>FPIVQVVGFQNSGKTTFIERILEKASEQGLNLGCLKHHGHGGEPQTFTEGKDTDRYQAAGADVTAVEGAGVLQLTARRLWDLTRLIELYQFLETDCLLIEGFKKAPYPKVVILSEKEDLEALKTVN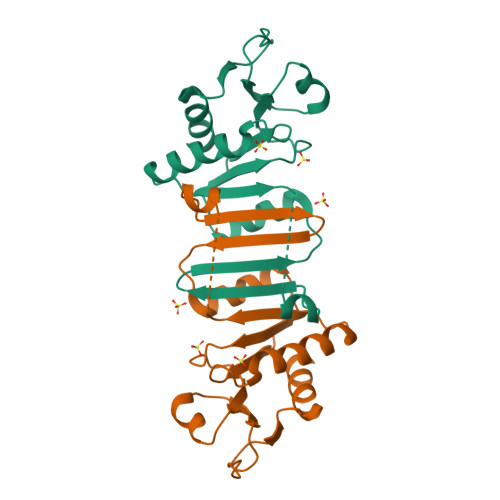TIAIIYRKKEHMTEHQGLPIFHADDPVAVDLVLSQLKGES[5x]>[2x]SGRHERDAFDTLFDHAPDKLNVVKKTLITFVNKHLNKL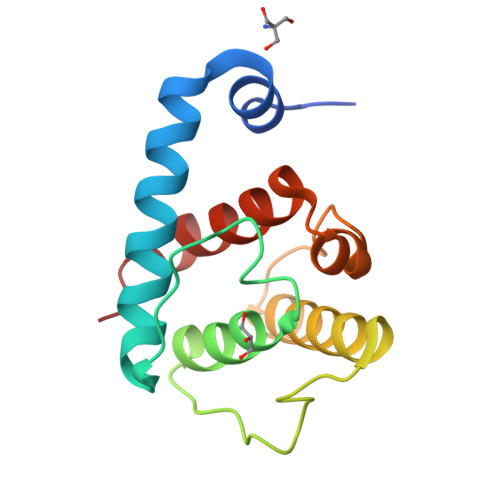NLEVTELETQFADGVYLVLLMGLLEGYFVPLHSFFLTPDSFEQKVLNVSFAFELMQDGGLEKPKPRPEDIVNCDLKSTLRVLYNLFTKYRNVE> MKRNDVILRTTTAVVTPIIVLFSVQ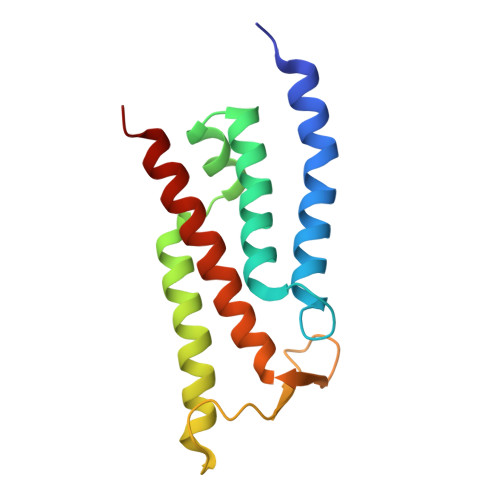LFFAGHYYPGGGFIGGLMTAGAIVLLLLAFDIETVRKMVPINYKWLVAIGLLFAVGTGMSSMFLDRPFLTHAYKYVHLPLLDHTSLHTAVLFDLGVYFVVVGVTMIIIETIGESD>[2x]RGSHHHHHHGSMAPSPEGVTVVLGAQWGDEGKGKLVDILAAEADICARCAGGNNAGHTIVVRNDKGEKTSYAF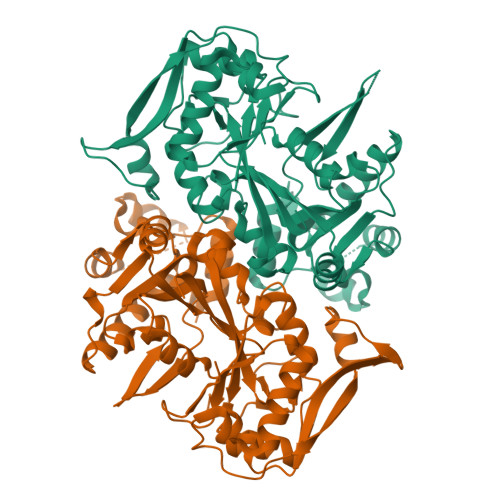NLLPSGLINPECTAFIGSGVVVHVPSLFNELDTLERKGLKVAGRLLVSDRAHLVMGFHQIVDGLKEVELGGSSIGTTRKGIGPAYSSKASRSGLRVHHLFDPTFPAKFRKLVEGRFKRYGHFEFDTEGEIEMYLAFAERLRPFIVDGPTFMHNALSSGKRVLVEGANALMLDLDYGTYPFVTSSSTSIGGVVSGLGISPFAIKRVVGVIKAYTTRVGGGPFPTEDLATVGETLQEVGAEYGTVTGRRRRCGWLDLVVMKYSTMINGYTSLNLTKLDVLDGFEEIKVATGYKIDGVEVEGFPADLDRLAKVEVQYATLPGWKTDISNCKTYEEFPENAKAYIKFIEDYLGVKVQYVGVGPGRDQNVIIF>GPLCAQEFSDLTDPLYIKKICLEKVPEWNHFTEDNLRVKQILSGLTNQLFEVGLKEETANNYNSIRTRVLFRIYGKHVDELYNTISEFEVYKTMSKYKIAPQLLNTFNGGRIEEWLYGDPLRIDDLKNPTILIGIANVLGKFHTLSRKRHLPEHWDRTPCIFKMMEKWKNQLFKYKNIEKYNCDIHKYIKESDKFIKFMKVYSKSDNLANTIVFCHNDLQENNIINTNKCLRLIDFEYSGFNFLATDIANFFIETSIDY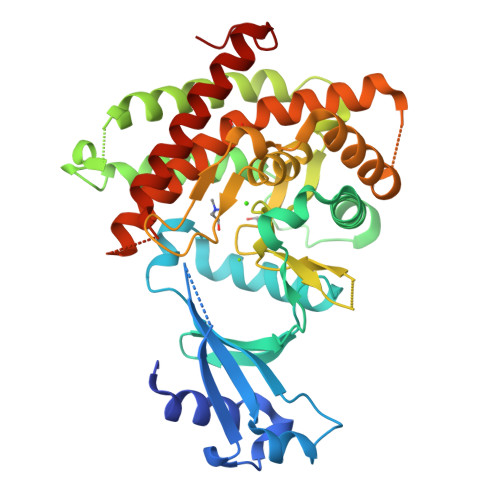SVSSYPFFEIDKKKYISYENRKLFITAYLSNYLDKSLVVPTPKLIDEILEAVEVQALGAHLLWGFWSIIRGYQTKSYNEFDFFLYAEQRLKMYDDQKEYLISNNIIKGYD[4x];> ENLYFQ> MSNGPEPHGNKIEQPEIRADERQDAGGPANGAPSTSGGAYSQGAKSGGQAAPDPSGSYGIKDAPVAPATIAFEFDGQQVEAQPGETIWAVAKRLGTHIPHLCHKPDPG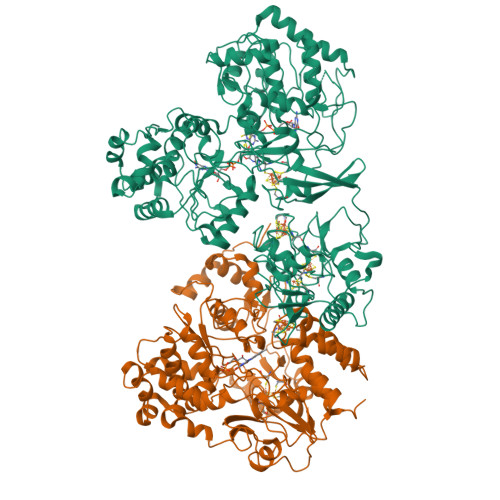YRPDGNCRACMVEIEGERVLAASCKRTPAIGMKVKSATERATKARAMVLELLVADQPERATSHDPSSHFWVQADVLDVTESRFPAAERWTSDVSHPAMSVNLDACIQCNLCVRACREVQVNDVIGMAYRAAGSKVVFDFDDPMGGSTCVACGECVQACPTGALMPAAYLDANQTRTVYPDREVKSLCPYCGVGCQVSYKVKDERIVYAEGVNGPANQNRLCVKGRFGFDYVHHPHRLTVPLIRLENVPKDANDQVDPANPWTHFREATWEEALDRAAGGLKAIRDTNGRKALAGFGSAKGSNEEAYLFQKLVRLGFGTNNVDHCTRLCHASSVAALMEGLNSGAVTAPFSAALDAEVIVVIGANPTVNHPVAATFLKNAVKQRGAKLIIMDPRRQTLSRHAYRHLAFRPGSDVAMLNAMLNVIVTEGLYDEQYIAGYTENFEALREKIVDFTPEKMASVCGIDAETLREVARLYARAKSSLIFWGMGVSQHVHGTDNSRCLIALALITGQIGRPGTGLHPLRGQNNVQGASDAGLIPMVYPDYQSVEKDAVRELFEEFWGQSLDPQKGLTVVEIMRAIHAGEIRGMFVEGENPAMSDPDLNHARHALAMLDHLVVQDLFLTETAFHADVVLPASAFAEKAGTFTNTDRRVQIAQPVVAPPGDARQDWWIIQELARRLDLDWNYGGPADIFAEMAQVMPSLNNITWERLEREGAVTYPVDAPDQPGNEIIFYAGFPTESGRAKIVPAAIVPPDEVPDDEFPMVLSTGRVLEHWHTGSMTRRAGVLDALEPEAVAFMAPKELYRLGLRPGGSMRLETRRGAVVLKVRSDRDVPIGMIFMPFCYAEAAANLLTNPALDPLGKIPEFKFCAARVVPAEAAPMAAEHHHHHH;> MSEASGTVRSFAHPGRGRNVARAVPKGRQVDPHAKVEIEELLGTRPRQRDLLIEHLHLIQDTYGQISADHLAALADEMSLAFAEVFETATFYAHFDVVKEGEADIPRLTIRVCDSITCAMFGADELLETLQRELASDAVRVVRAPCVGLCDHAPAVEVGHNFLHRADLASVRAAVEAEDTHAHIPTYVDYDAYRAGGGYATLERLRSGELPVDDVLKVLDDGGLRGLGGAGFPTGRKWRSVRGEPGPRLMAVNGDEGEPGTFKDQLYLNTDPHRFLEGMLIGAHVVEAADVYIYLRDEYPISREILAREIAKLPEGGTRIHLRRGAGAYICGEESSLIESLEGKRGLPRHKPPFPFQVGLFNRPTLINNIETLFWVRDLIERGAEWWKSHGRNGRVGLRSYSVSGRVKEPGVKLAPAGLTIQELIDEYCGGISDGHSFAAYLPGGASGGILPASMNDIPLDFGTLEKYGCFIGSAAVVILSDQDDVRGAALNLMKFFEDESCGQCTPCRSGTQKARMLMENGVWDTDLLGELAQCMRDASICGLGQAASNPVSTVIKYFPDLFPEPRAVAAE> MGSVTPIPLPKIDEPEEYNTNYILFWNHVGLELNRVTHTVGGPLTGPPLSARALGMLHLAIHDAYFSICPPTDFTTFLSPDTENAAYRLPSPNG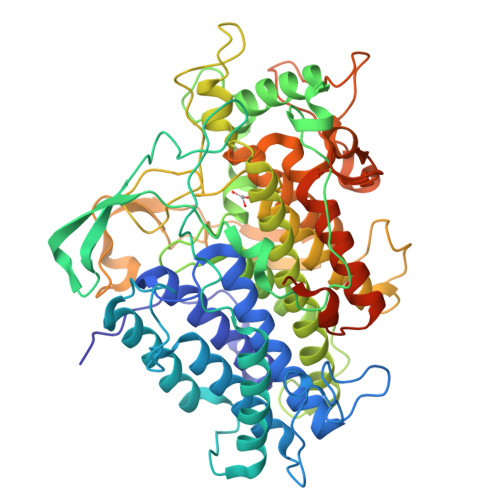ANDARQAVAGAALKMLSSLYMKPVEQPNPNPGANISDNAYAQLGLVLDRSVLEAPGGVDRESASFMFGEDVADVFFALLNDPRGASQEGYNPTPGRYKFDDEPTHPVVLIPVDPNNPNGPKMPFRQYHAPFYGKTTKRFATQSEHFLADPPGLRSNADETAEYDDAVRVAIAMGGAQALNSTKRSPWQTAQGLYWAYDGSNLIGTPPRFYNQIVRRIAVTYKKEEDLANSEVNNADFARLFALVDVACTDAGIFSWKEKWEFEFWRPLSGVRDDGRPDHGDPFWLTLGAPATNTNDIPFKPPFPAYPSGHATFGGAVFQMVRRYYNGRVGTWKDDEPDNIAIDMMISEELNGVNRDLRQPYDPTAPIEDQPGIVRTRIVRHFDSAWELMFENAISRIFLGVHWRFDAAAARDILIPTTTKDVYAVDNNGATVFQNVEDIRYTTRGTREDEEGLFPIGGVPLGIEIADEIFNNGLKPTPPEIQPMPQETPVQKPVGQQPVKGMWEEEQAPVVKEAP Phosphoethanolamine (pEtN) cellulose is a naturally occurring modified cellulose produced by several Enterobacteriaceae. The minimal components of the E. coli cellulose synthase complex include the catalytically active BcsA enzyme, a hexameric semicircle of the periplasmic BcsB protein, and the outer membrane (OM)-integrated BcsC subunit containing periplasmic tetratricopeptide repeats (TPR). Additional subunits include BcsG, a membrane-anchored periplasmic pEtN transferase associated with BcsA, and BcsZ, a periplasmic cellulase of unknown biological function. Cellulose is a common bacterial biofilm component produced by a variety of prokaryotes, such as Escherichia coli (Ec), Salmonella enterica, and Gluconacetobacter/Komagataeibacter xylinus (Gx). These Gram-negative bacteria synthesize cellulose and secrete it across the cell envelope via the Bacterial cellulose synthase (Bcs) complex.

To improve the resolution of the BcsB-BcsC complex map, BcsC’s TPR#1–4 were fused to the N-terminus of BcsB, after its N-terminal signal sequence and separated by a linker. As also observed for the wild type Bcs complex, cryo-EM analysis identified a fully assembled Bcs complex together with (likely dissociated) partial subcomplexes containing three to five BcsB protomers. Although additional BcsC density similar to the one described above was also observed in a fully assembled complex, the highest quality map revealing the BcsB-BcsC interaction was obtained for a tetrameric BcsB assembly. TPR#1 mediates all interactions with BcsB and is best resolved. TPR#2 is rotated by about 45° relative to TPR#1 and extends away from BcsB. In complex with BcsB, TPR#1 is oriented with its interhelical loop pointing towards the center of the BcsB semicircle. It interacts extensively with one side of CBD-1’s jelly roll, as well as the region connecting the jelly roll with FD-1 (residues 208–220), Fig. 3b. In particular, TPR#1’s N-terminal helix (helix-1) rests on a short helical segment of a CBD-1 loop, such that its Gln30, Gln34, and Leu37 stack on top of BcsB’s Leu162, Phe163, and Ile164. The helix’s C-terminal end fits into a hydrophobic pocket formed by the CBD-1/FD-1 connection. Due to this arrangement, the observed BcsB-BcsC interaction is only possible with the last subunit of the BcsB hexamer.

> AWSHPQFEKVEAAPTAQQQLLEQVRLGEATHREDLVQQSLYRLELIDPNNPDVVAARFRSLLRQGDIDGAQKQLDRLSQLAPSSNAYKSSRTTMLLSTPDGRQALQQARLQATTGHAEEAVASYNKLFNGAPPEGDIAVEYWSTVAKIPARRGEAINQLKRINADAPGGSGSGSGVQGADAPVVAQNGPSRDVKLTFAQIAPPPGSMVLRGINPNGSIEFGMRSDEVVTKAMLNLEYTPSPSLLPVQSQLKVYLNDELMGVLPVTKEQLGKKTLAQMPINPLFISDFNRVRLEFVGHYQDVCEKPASTTLWLDVGRSSGLDLTYQTLNVKNDLSHFPVPFFDPSDNRTNTLPMVFAGAPDVGLQQASAIVASWFGSRSGWRGQNFPVLYNQLPDRNAIVFATNDKRPDFLRDHPAVKAPVIEMINHPQNPYVKLLVVFGRDDKDLLQAAKGIAQGNILFRGESVVVNEVKPLLPRKPYDAPNWVRTDRPVTFGELKTYEEQLQSSGLEPAAINVSLNLPPDLYLMRSTGIDMDINYRYTMPPVKDSSRMDISLNNQFLQSFNLSSKQEANRLLLRIPVLQGLLDGKTDVSIPALKLGATNQLRFDFEYMNPMPGGSVDNCITFQPVQNHVVIGDDSTIDFSKYYHFIPMPDLRAFANAGFPFSRMADLSQTITVMPKAPNEAQMETLLNTVGFIGAQTGFPAINLTVTDDGSTIQGKDADIMIIGGIPDKLKDDKQIDLLVQATESWVKTPMRQTPFPGIVPDESDRAAETRSTLTSSGAMAAVIGFQSPYNDQRSVIALLADSPRGYEMLNDAVNDSGKRATMFGSVAVIRESGINSLRVGDVYYVGHLPWFERVWYALANHPILLAVLAAISVILLAWVLWRLLRIISRRRLNPDNE> TGGTGGTGGTGGTTGTGGTGGTG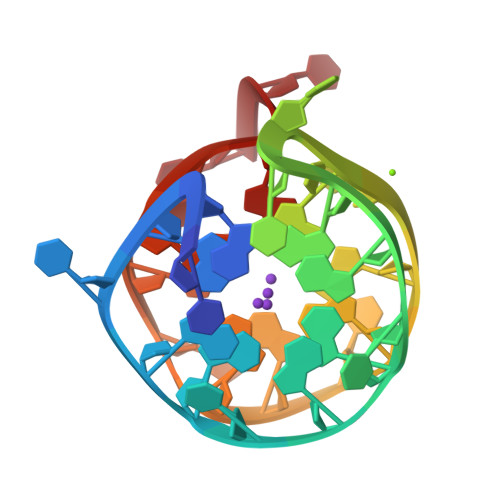GTGTT Inositol hexakisphosphate kinases (IP6Ks) are emerging as relevant pharmacological targets because a multitude of disease-related phenotypes has been associated with their function. Genetic knockouts of the three mammalian inositol hexakisphosphate kinase (IP6K) isozymes – enzymes involved in PP-InsP biosynthesis – have revealed their involvement in distinct biological processes, including insulin signaling, apoptosis, cancer metastasis, and lifespan regulation in mice. Here, we implemented the analog-sensitive approach for IP6Ks to identify isozyme-selective inhibitors. While the exact structures of mammalian IP6Ks have remained elusive to date, those of other members of the InsP kinase family, for example Homo sapiens IPMK and Entamoeba histolytica IP6KA, have successfully been deciphered.

However, the evolutionarily related ortholog IP6KA from Entamoeba histolytica (Eh) was sensitized to inhibition by FMP-201300 when its methionine gatekeeper was mutated to valine. The approach therefore appears transferable not only between the mammalian isozymes, but also to other IP6K orthologs. However, to date the mammalian IP6K isozymes have been recalcitrant in crystallization efforts. This limitation may, in part, be circumvented by focusing on EhIP6KA, which has been crystallized and structurally analyzed. An alignment of the AlphaFold structure model of IP6K1 and the crystal structure of EhIP6KA suggests significant structural conservation, especially within the active site. The fact that FMP-201300 recapitulates its gatekeeper mutant selectivity and allosteric binding mode against EhIP6KAM85V prompted us to attempt co-crystallization of this related kinase and the inhibitor. While the valine gatekeeper mutant of EhIP6KA was readily crystallized using the published conditions for the WT counterpart, soaking or co-crystallization with FMP-201300 remained unsuccessful. Remarkably, the structures of the WT and mutant EhIP6KA are virtually identical except for the additional space generated by the reduced gatekeeper size. This result illustrates a potential limitation of crystallography, as it can only provide a snapshot of a momentary protein conformation and may not be suited to unveil subtle dynamic changes that occur upon inhibitor binding. The fact that the inhibitor exhibits the same behavior against IP6K2 and EhIP6KA diminishes the likelihood of a distant allosteric site, since IP6K1 and IP6K2 only share 47% sequence identity, most of which lies within the catalytic region. After an InsP6-competitive mode of action had been ruled out, attempts to gain structural insights by crystallographic analysis of the ortholog EhIP6KA were undertaken.

> GSFTQQLHPDGQYLLKPCLSHRERDFYLHIKDDKEWTGTGIIPKFYGVELHEFGFGELEFIRVENLMYKYKRPFVLDLKIGTQTWDPETASSKMKKRLVVDSTSTTTSLGVRFSGMERNIGEEKPILYSRYLCTHEVNTRDSLKEYIKLFFNDGKKYRKELVPYFISQLDKMIEVMKKREYKMFSSSVLFVYDSTTTLEDKKYNCKMIDFAHNWILSEEECTVEDGFLFGLNNLKSILEDIENEFKSL>MDITELLAFSAKQGASDLHLSAGLPPMIRVDGDVRRINLPPLEHKQVHALIYDIMNDKQRKDFEEFLETDFSFEVPGVARFRVNAFNQNRGAGAVFRTIPSKVLTMEELGMGEVFKRVSDVPRGLVLVTGPTGSGKSTTLAAMLDYLNNTKYHHILTIEDPIEFVHESKKCLVNQREVHRDTLGFSEALRSALRE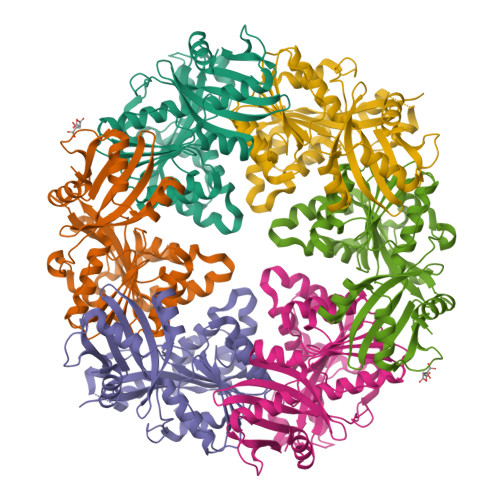DPDIILVGEMRDLETIRLALTAAETGHLVFGTLHTTSAAKTIDRVVDVFPAEEKAMVRSMLSESLQSVISQTLIKKIGGGRVAAHEIMIGTPAIRNLIREDKVAQMYSAIQTGGSLGMQTLDMCLKGLVAKGLISRENAREKAKIPENFGAAALEHHHHHH[3x]>MKALSFLTPIVTLALVAGAFASVGPVANLKIGNAAVSPDGYTRDAVVVNGATPGPLIVGNKGDNFRLNVIDELTNHTMLKSTSIHWHGFFQHGTNWADGGAFVNQCPISSGHSFSYNFQAKDQAGTFWYHSHLSTQYCDGLRGPFVVYDPKDPHKKLYDVDNESTVITLEDWYHTAARLGPRFP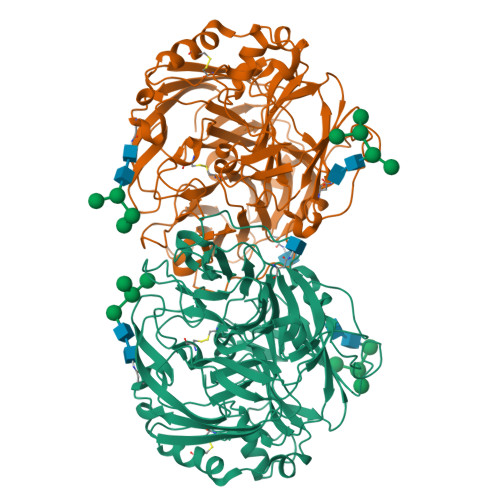LGSDSTLINGLGRSATTATGDLAVIKVTRGKRYRFRLVSLSCDPFYTFSIDGHNMTIIEADAVNTKPHTVDSLEIFAGQRYSFILNANQPVDNYWVRANPNFGNVGFTNGINSAILRYDGAAVAEPATAIPPASVTPLLETDLHPLVSTPVPGSPVAGGVDKALNFVFNFDGTNFFINDATFTPPSVPVLLQILSGAQAAQDLLPSGSVIPLPALSTIELSFPATANAPGVPHPFHLHGHTFAVVRSAGSTAYNYEDPVWRDVVSTGTPAAGDNVTIRFVTDNPGPWFLHCHIDFHLEAGFAVVFAEDLPGTPAANPVPQSWSDLCPIYDALAEDDQ[2x]N-(2-phenylethyl)quinazolin-4-amine | C16 H15 N3 | 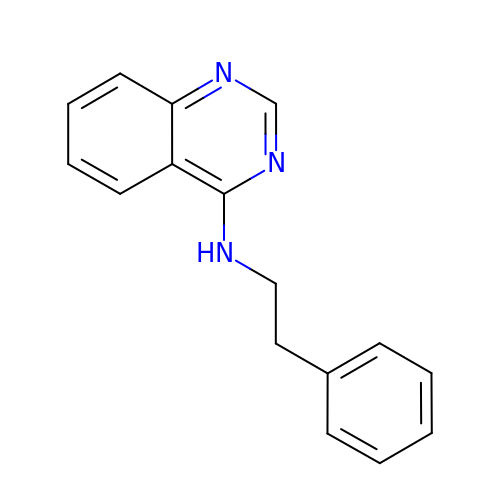YKOSADJQCBRMRR-UHFFFAOYSA-N> GPMDQQNSAVIGQLRLELQQARTEVETADKWRLEC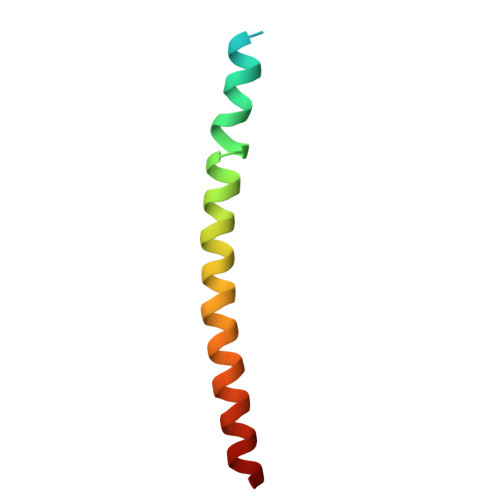IDVCSVLTNRLEEEAGFLNSLLK> SNAIAEKGEKLYHMMMNKKVNLIKDRRRKLSTVPKCFLGNEFVAWLLEIGEISKTEEGVNLGQALLENGIIHHVSD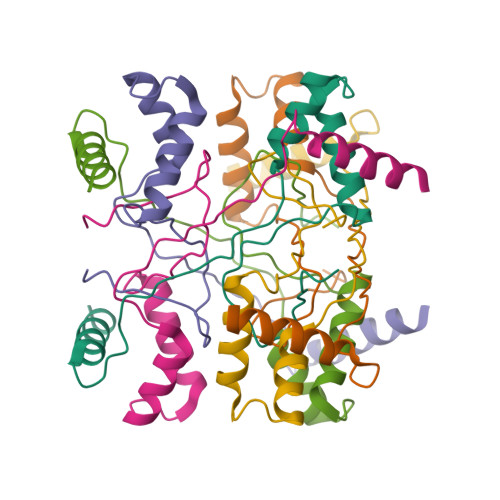KHQFKNEQVMYRFRYDDG>[2x]GMAPPSVFAEVPQAQPVLVFKLIADFREDPDPRKVNLGVGAYRTDDCQPWVLPVVRKVEQRIANNSSLNHEYLPILGLAEFRT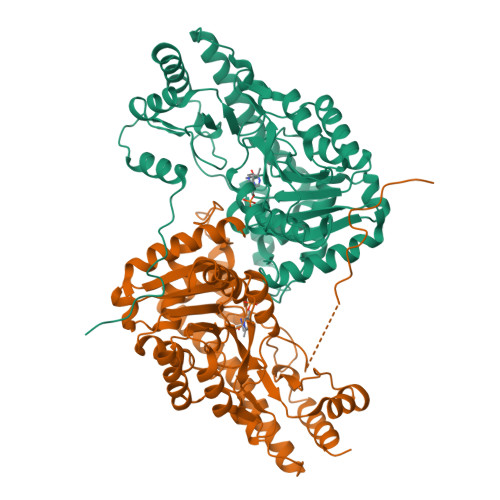CASRLALGDDSPALQEKRVGGVQSLGGTGALRIGAEFLARWYNGTNNKDTPVYVSSPTWENHNGVFTTAGFKDIRSYRYWDTEKRGLDLQGFLSDLENAPEFSIFVLHACAHNPTGTDPTPEQWKQIASVMKRRFLFPFFDSAYQGFASGNLEKDAWAIRYFVSEGFELFCAQSFSKNFGLYNERVGNLTVVAKEPDSILRVLSQMQKIVRVTWSNPPAQGARIVARTLSDPELFHEWTGNVKTMADRILSMRSELRARLEALKTPGTWNHITDQIGMFSFTGLNPKQVEYLINQKHIYLLPSGRINMCGLTTKNLDYVATSIHEAVTKIQ>SMAGAARSLSRFR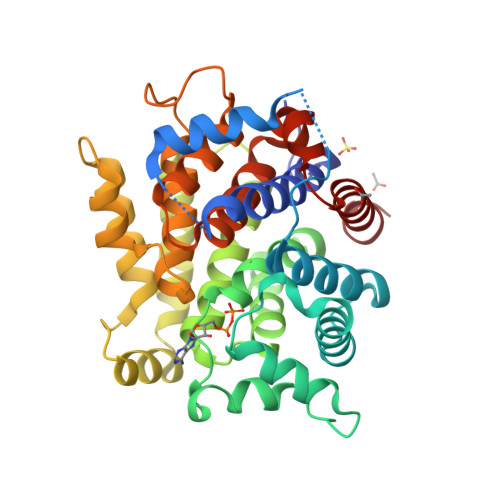GCLAGALLGDCVGSFYEAHDTVDLTSVLRHVQSLEPDPGTPGSERTEALYYTDDTAMARALVQSLLAKEAFDEVDMAHRFAQEYKKDPDRGYGAGVVTVFKKLLNPKCRDVFEPARAQFNGKGSYGNGGAMRVAGISLAYSSVQDVQKFARLSAQLTHASSLGYNGAILQALAVHLALQGESSSEHFLKQLLGHMEDLEGDAQSVLDARELGMEERPYSSRLKKIGELLDQASVTREEVVSELGNGIAAFESVPTAIYCFLRCMEPDPEIPSAFNSLQRTLIYSISLGGDTDTIATMAGAIAGAYYGMDQVPESWQQSCEGYEETDILAQSLHRVFQKS[2x]> MEGISIYTSDNYTEEMGSGDYDSMKEPCFREENANFNKIFLPTIYSIIFLTGIVGNGLVILVMGYQKKLRSMTDKYRLHLSVADLLFVITLPFWAVDAVANWYFGNFLCKAVHVIYTVNLYSSVLILAFISLDRYLAIVHATNSQRPRKLLAEKVVYVGVWIPALLLTI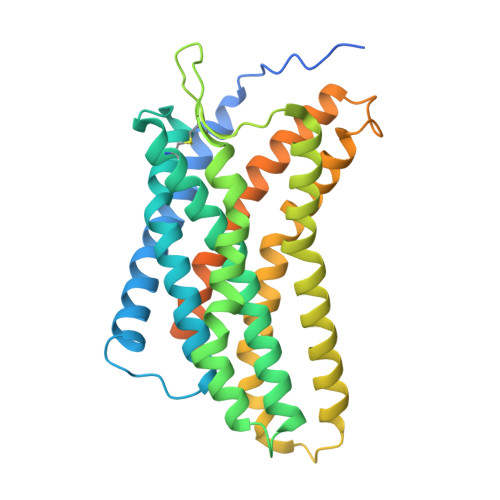PDFIFANVSEADDRYICDRFYPNDLWVVVFQFQHIMVGLILPGIVILSCYCIIISKLSHSKGHQKRKALKTTVILILAFFACWLPYYIGISIDSFILLEIIKQGCEFENTVHKWISITEALAFFHCCLNPILYAFLGAKFKTSAQHALTSVSRGSSLKILSKGKRGGHSSVSTESESSSFHSSDYKDDDDK>GSPGLKGDKGIPGDKGAKGESGLPDVASLRQQVEALQGQVQHLQAAFSQYKKVELFPNGQSVGEKIFKTAGFVKPFTEAQLLCTQAGGQLASPRSAAENAALQQLVVAKNEAAFLSMTDSKTEGKFTYPTGESLVYSNWAPGEPNDDGGSEDCV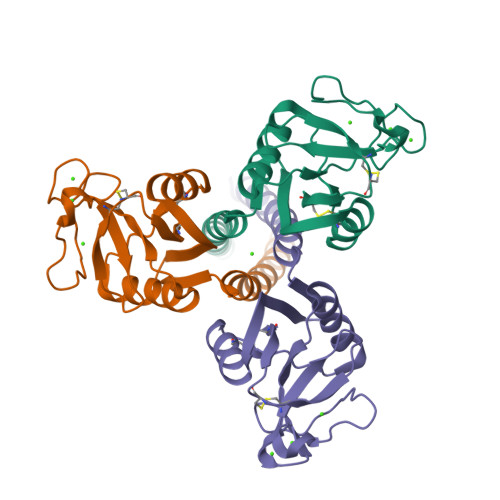EIFTNGKWNDRACGEKRLVVCEF[3x]>VEIPSSFDSRKKWPRCKSIATIRDQSRCGSCWAFGAVEAMSDRSCIQSGGKQNVELSAVDLLSCCESCGLGCEGGILGPAWDYWVKEGIVTGSSKENHAGCEPYPFPKCEHHTKGKYPPCGSKIYKTPRCKQTCQKKYKTPYTQDKHRGKSSYNVKNDEKAIQKEIMKYGPVEAGFTVYEDFLNYKSGIY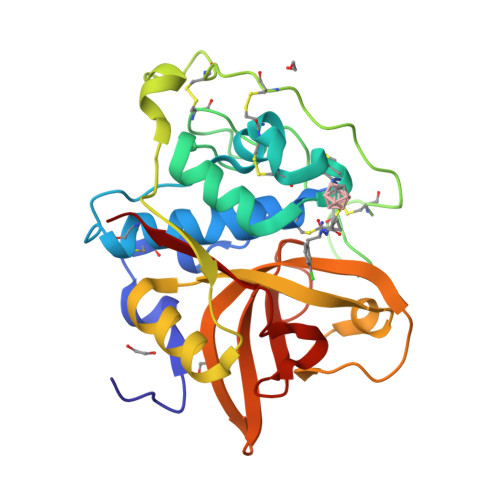KHITGETLGGHAIRIIGWGVENKAPYWLIANSWNEDWGENGYFRIVRGRDECSIESEVTAGRIN[3x]>[2x]MAHHHHHHMPRITQEISYNCDYGDNTFNLAIDIGGTLAKVVFSPIHSNRLMFYTIETEKIDKFMELLHSIIKEHNNGCYRMTHIIATGGGAFKFYDLLYENFPQIKGISRFEEMEGLIHGLDFFIHEIPDEVFTYNDQDGERIIPTSSGTMDSKAIYPYLLVNIGSGVSILKVTEPNNFSRVGGSSLGGGTLWGLLSLITGAQTYDQMLDWAQEGDNSSVDMLVGDIYGTDYNKIGLKSSAI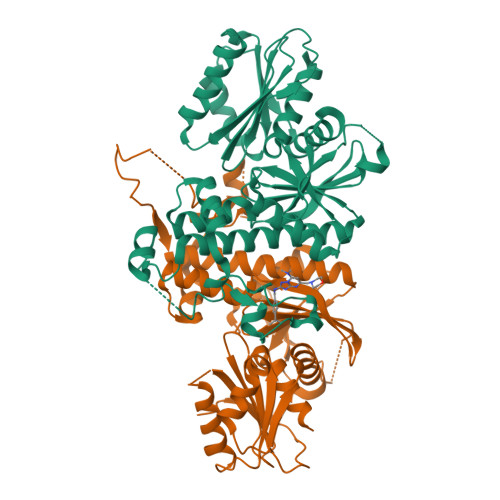ASSFGKVFQNRMTSNKSLENNENKLYSSHESIEKNNGQMFKNPDICKSLLFAISNNIGQIAYLQAKINNIQNIYFGGSYTRGHLTTMNTLSYAINFWSQGSKQAFFLKHEGYLGAMGAFLSASRHSSTKKTST> ADKLFINALKKKFEESPEEKKTTFYTLGGWKQSER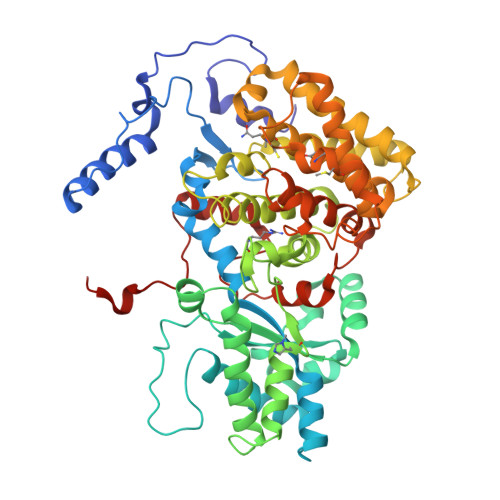KTEFVNAGKEVAAKRGIPQYNPDIGTPLGQRVLMPYQVSTTDTYVEGDDLHFVNNAAMQQMWDDIRRTVIVGLNHAHAVIEKRLGKEVTPETITHYLETVNHAMPGAAVVQEHMVETHPALVADSYVKVFTGNDEIADEIDPAFVIDINKQFPEDQAETLKAEVGDGIWQVVRIPTIVSRTCDGATTSRWSAMQIGMSMISAYKQAAGEAATGDFAYAAKHAEVIHMGTYLPVRRARGENEPGGVPFGYLADICQSSRVNYEDPVRVSLDVVATGAMLYDQIWLGSYMSGGVGFTQYATAAYTDNILDDFTYFGKEYVEDKYGLCEAPNNMDTVLDVATEVTFYGLEQYEEYPALLEDQFGGSQRAAVVAAAAGCSTAFATGNAQTGLSGWYLSMYLHKEQHSRLGFYGYDLQDQCGASNVFSIRGDEGLPLELRGPNYPNYAMNVGHQGEYAGISQAPHAARGDAFVFNPLVKIAFADDNLVFDFTNVRGEFAKGALREFEPAGERALITPA> SGWVWNQFFVIEEYTGPDPVLVGRLHSDIDSGDGNIKYILSGEGAGTIFVIDDKSGNIHATKTLDREERAQYTLMAQAVDRDTNRPLEPPSEFIVKVQDINDNPPEFLHEIYHANVPERSNVGTSVIQVTASDADDPTYGNSAKLVYSILEGQPYFSVEAQTGIIRTALPNMDREAKEEYHVVIQAKDMGGHMGGLSGTTKVTITL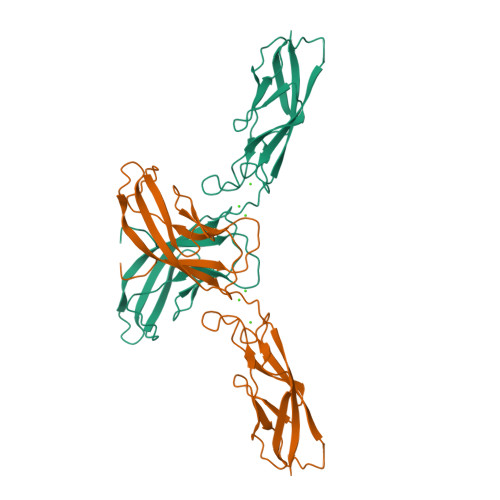TDDYKDDDK{1,3-PHENYLENEBIS[IMINO(2-OXOETHANE-2,1-DIYL)]}BIS(PHOSPHONIC 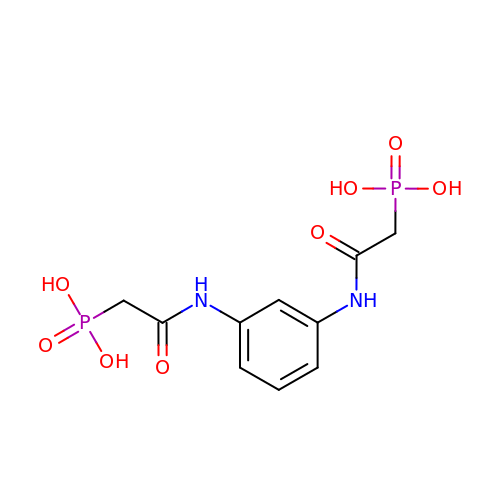ACID) | C10 H14 N2 O8 P2 | BHGKTXYPXMTFLT-UHFFFAOYSA-N> KGLGKGGA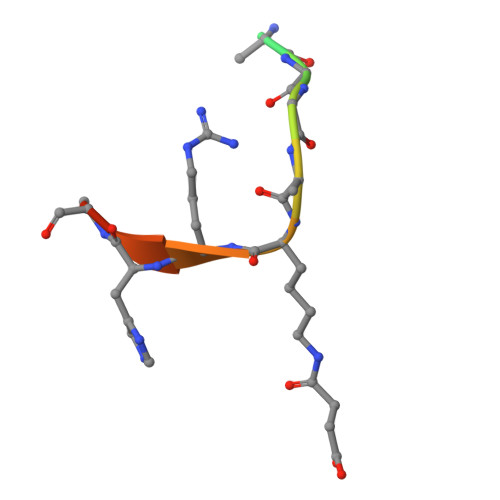XRHRKW>[2x]PPYTVVYFPVRGRCAALRMLLADQGQSWKEEVVTVETW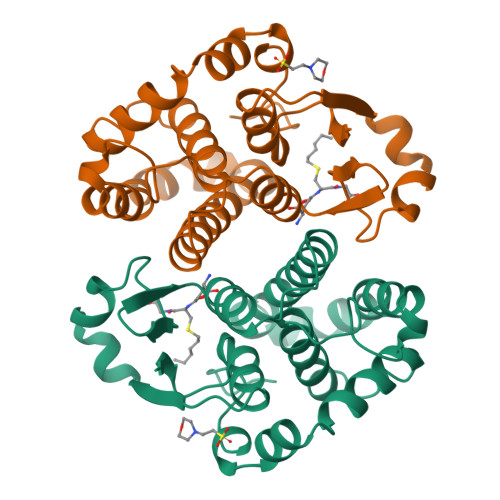QEGSLKASCLYGQLPKFQDGDLTLYQSNTILRHLGRTLGLYGKDQQEAALVDMVNDGVEDLRCKYISLIFTNYEAGKDDYVKALPGQLKPFETLLSQNQGGKTFIVGDQISFADYNLLDLLLIHEVLAPGCLDAFPLLSAYVGRLSARPKLKAFLASPEYVNLPINGNGKQ> GAMGATPEEYYKATGKKITEYHESPMLTKLVEEGKLPPVEQRLPEEPLVVQPVEKVGQFGGTWRRVWKGPSDRWGISKLIEVKLAFWDKEGGKLVPGLAKSWEVLENGRVYIFHLRKGVKWSDGAPYTAHDIVFWVNDIVGNDDITPSKPDWYNIGVKVEALDDYTVKFEFSKPYGLFLLKVPYGGFTGAPAHYLKQFHPKYTPMEEIEKKMVEGVHNTWVDLFNDKNDFLENTELPTLSPWKPITDPTEQFYILERNPYFWAVDIEGNQLPYIDYVRHEYVKNDEVILLKAISGEIDMQWRHIGGLGAGAGNFTLLMENSQSGGYRVLKWIAANGSASRISLNYAHSDEVLRKVFNDVRFRQALSLAINREEINEILFNGLAEPRQASLVSGSPYFDPEWEKAYAEYDPDRANKLLDEMGLKWDDKHEYRLLPDGRPLRFT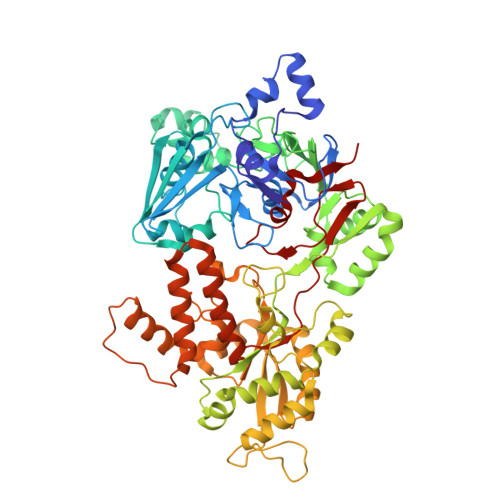ITVTGQFHVDVWTMVKEYWKQIGVWVEIENLERSLFYERADAGDFDAMVWNMDRAAQPLSSPMVIFPGSENIADFWYIGWSGWISYYIDKNIRGVEPEEVPEGPEPPEVVYRLVDLYYQIASTPDPDKIKELMAEATKIHRENLWMIGTVGEDLSPAIAKNNFRNVPEFLVTDDVLRTPLNAMPMQFFIEQ>[2x]GSHMNAAAEAEFNILMATDSYKVTHYKQYPPNTSKVYSYFECREKKTENSKVRKVKYEETVFYGLQYILN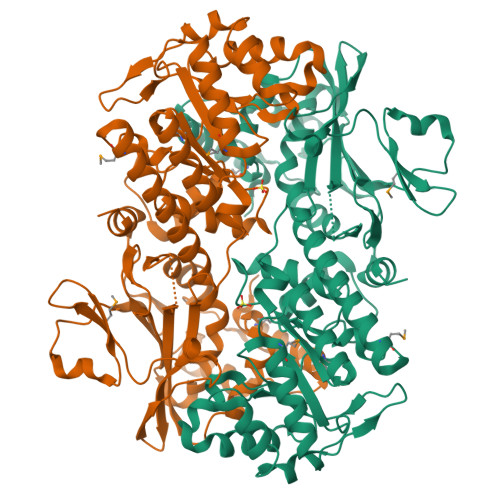KYLKGKVVTKEKIQEAKEVYREHFQDDVFNERGWNYILEKYDGHLPIEVKAVPEGSVIPRGNVLFTVENTDPECYWLTNWIETILVQSWYPITVATNSREQKKILAKYLMETSGNLDGLEYKLHDFGYRGVSSQETAGIGASAHLVNFKGTDTVAGIALIKKYYGTKDPVPGYSVPAAEHSTITAWGKDHEKDAFEHIVTQFSSVPVSVVSDSYDIYNACEKIWGEDLRHLIVSRSTEAPLIIRPDSGNPMDTVLKVLDILGKKFPVTENSKGYKLLPPYLRVIQGDGVDINTLQEIVEGMKQKKWSIENVSFGSGGALLQKLTRDLLNCSFKCSYVVTNGLGVNVFKDPVADPNKRSKKGRLSMHRTPAGNFVTLEEGKGDLEEYGHDLLHTVFKNGKVTKSYSFDEVRKNAQLNIEQDVAPH>[3x]MWKRSEQMKIKSGKCNMAAAMETEQLGVEIFETADCEENIESQDRPKLEPFYVERYSWSQLKKLLADTRKYHGYMMAKAPHDFMFVKRNDPDGPHSDRIYYLAMSGENRENTLFYSEIPKTINRAAVLMLSWKPLLDLFQATLDYGMYSREEELLRERKRIGTVGIASYDYHQGSGTFLFQAGSGIYHVKDGGPQGFTQQPLRPNLVETSCPNIRMDPKLCPADPDWIAFIHSNDIWISNIV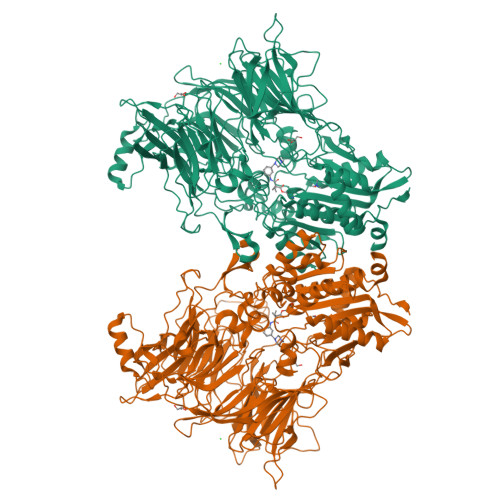TREERRLTYVHNELANMEEDARSAGVATFVLQEEFDRYSGYWWCPKAETTPSGGKILRILYEENDESEVEIIHVTSPMLETRRADSFRYPKTGTANPKVTFKMSEIMIDAEGRIIDVIDKELIQPFEILFEGVEYIARAGWTPEGKYAWSILLDRSQTRLQIVLISPELFIPVEDDVMERQRLIESVPDSVTPLIIYEETTDIWINIHDIFHVFPQSHEEEIEFIFASECKTGFRHLYKITSILKESKYKRSSGGLPAPSDFKCPIKEEIAITSGEWEVLGRHGSNIQVDEVRRLVYFEGTKDSPLEHHLYVVSYVNPGEVTRLTDRGYSHSCCISQHCDFFISKYSNQKNPHCVSLYKLSSPEDDPTCKTKEFWATILDSAGPLPDYTPPEIFSFESTTGFTLYGMLYKPHDLQPGKKYPTVLFIYGGPQVQLVNNRFKGVKYFRLNTLASLGYVVVVIDNRGSCHRGLKFEGAFKYKMGQIEIDDQVEGLQYLASRYDFIDLDRVGIHGWSYGGYLSLMALMQRSDIFRVAIAGAPVTLWIFYDTGYTERYMGHPDQNEQGYYLGSVAMQAEKFPSEPNRLLLLHGFLDENVHFAHTSILLSFLVRAGKPYDLQIYPQERHSIRVPESGEHYELHLLHYLQENLGSRIAALKVI~{N}-(3-chlorophenyl)-4-oxidanylidene-chromene-3-carboxamide 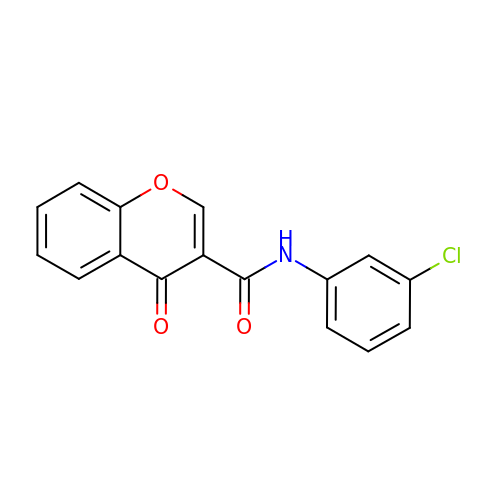| C16 H10 Cl N O3 | CVLFPXGWUQAEEW-UHFFFAOYSA-N> GPGSDDEINAQSVWSEEISSNYPLCIKNLMEGLKKNHHLRYYGRQQLSLFLKGIGLSADEALKFWSEAFTRNGNMTMEKFNKEYRFSFRHNYGLEG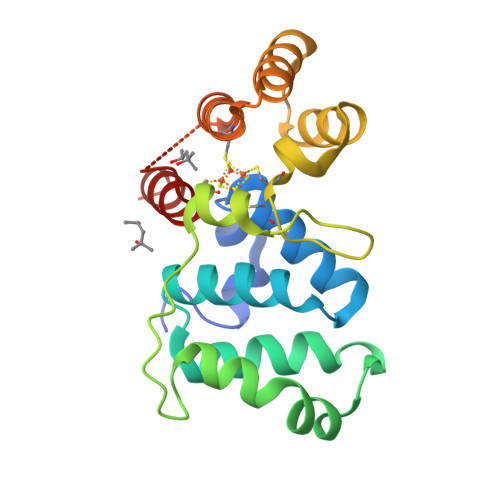NRINYKPWDCHTILSKPRPGRGDYHGCPFRDWSHERLSAELRSMKLTQAQIISVLDSCQKGEYTIACTKVFEMTHNSASADLEIGEQTHIAHPNLYFERSRQLQK>MTDKSQQFASDNYSGICPEAWAAMEKANHGHDRAYGDDQWTERASEYFRNLFETDCEVFFAFNGTAANSLALASLCQSYHSVICSETAHVETDECGAPEFFSNGSKLLTAASVNGKLTPQSIREVALKRQDIHYPKPRVVTITQATEVGTVYRPDELKAISATCKELGLNLHMDGARFTNACAFLGCSPAELTWKAGVDVLCFGGTKNGMAVGEAILFFNRQLAEDFDYRCKQAGQLASKMRFLSAPWVG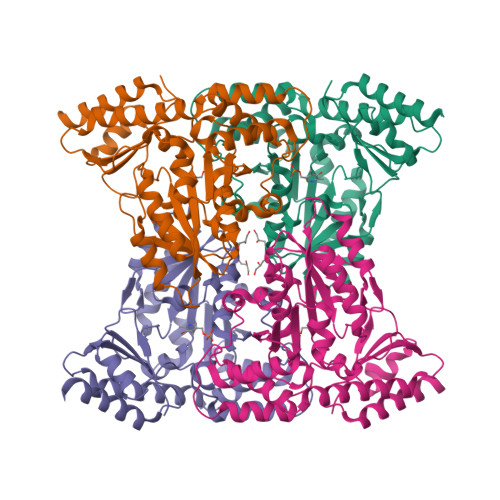LLEDGAWLRHGNHANHCAQLLALLVSDLPGVELMFPVEANGVFLQMPEHAIEALRAKGWRFYTFIGSGGARFMCSWDTEEERVRELAADIRSIITA[4x]> RRTDALTASPGR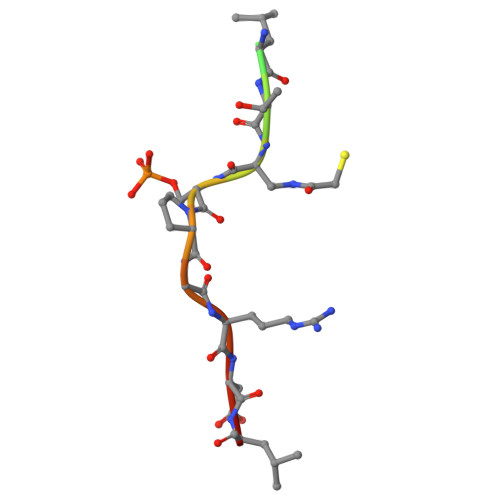DLP> DLD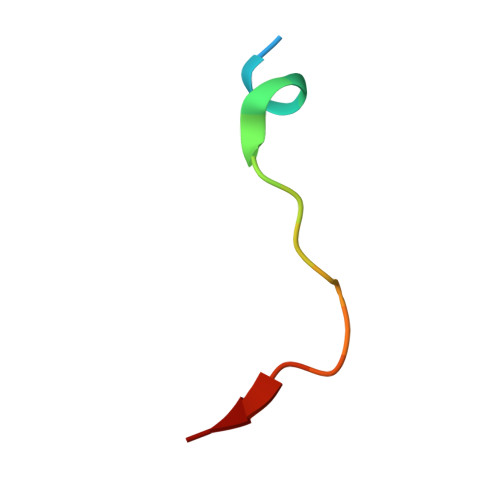LEMLAPYIPMDDDFQL>MGFKSWITEKLNPGQRIIRDMEPVSHRTNRKPFTTGQAYSKIEILNRTANMVIDSAAECSYTVGDKYNIVTYANGVKTKTLDTLLNVRPNPFMDISTFRRLVVTDLLFEGCAYIYWDGTSLYHVPAALMQVEADANKFIKKFIFNNQINYRVDEIIFIKDNSYVCGTNSQISGQSRVATVIDSLEKRSKMLNFKEKFLDNGTVIGLILETDEILNKKLRERKQEELQLDYNPSTGQSSVLILDGGMKAKPYSQISSFKDLDFKEDIAGFNKSICLAFGVPQVLIDGGNNANIRPNIELFYYMTIIPMLNKLTSSLTFFFGYKITPNTKEVAALTPDKEAEAKHLTSLVNNGIMTGNEARLELNLEPLDDEQMNRIRIPANVAGSATGVSGQEGGRPQGSTEGDKE[4x];>[4x]MQIITAEDYRLYGGLKRPELESGVEMMITAANALITSLLGMDDADAVDQLINTKPTRKKYFLSSPSATSVTKMTINDKEIDPEQYKLYSDGVILLKFSPPEGYMDVEYTQGGFNPIPEDLKLAACMLVDHWHKQDYRQAKTIGGETVTFNNTKSGIPEHIRTIIEVYRRV;>[2x]MDHRTSIAQALVDRIAQQMDGSQPDEYFNNLYGNVSRQTYKFEEIREFPYVAVHIGTETGQYLPSGQQWMFLELPILVYDKEKTDIQEQLEKLVADIKTVIDTGGNLEYTVSKPNGSTFPCEATDMSITSVSTDEGLLAPYGLAEINVTVRYQPPRRSLRR;> MTDKLIRELLIDVKQKGATRTAKSIENVSDALENAAAASELTNEQLGKMPKTLYSIERAADRAAKSLTKMQASRGMAGITKSIDSIGAKLDDLSIAMIEVADKLEAGFDGVSRSVKVMGNDVAAATEKVQDRLYDTNRVLGGTARGFNDTAGAAGRASRAIGNTSGSARGATRDFAAMAKVGGGLPLLYAAIASNIFVLQSAFEQLKLGDQLNRLEEFGVIVGTQTGTPVQSLARSLQEAAGYAISFEEAMRQASSASAYGFDAEQLNKFGLVARRAAAVLGVDMTDALNRVIKGVSKQEIELLDELGVTIRLNDAYADYVKQLNAANTGITYNINSLTTFQKQQAYANAVIAESTKRFGYLDEVLRATPWEQFAANADAALRTIQQAAAKYLGPVIDAINTVFYTSQASISAEAARAQEQTNKQIDPTNVGAVALSLSASEEGYNKALDMYKESLDKRNKLKSEFDKRMEQADFYTKLAIRQVGEGIPAGLATAGASEANKKFVEETAAMGLQVARLDKEVTDSTENLNAWKSAYQAAGAAAAKANPEFQKQINLQRDTTDPGAVYDFNSTVLKGLTEQQKAYNQTKKTASDLANDIQNVAQNTDTAAKTSATLADAIKNIESLSLGTGKSADEYVKNLNLGYNTLSEMKTASQALSEYVKLTGNETKNQLAVQQKIADVYNQTKDKEKAQEAGRRLELQQLEEQEAALRRVLQTNQGNKAVEREIEKIQLEKIKLTNQGMEAQKKVKDYTDKILGVDREIALLNNRTMTDTQYRLAQLNL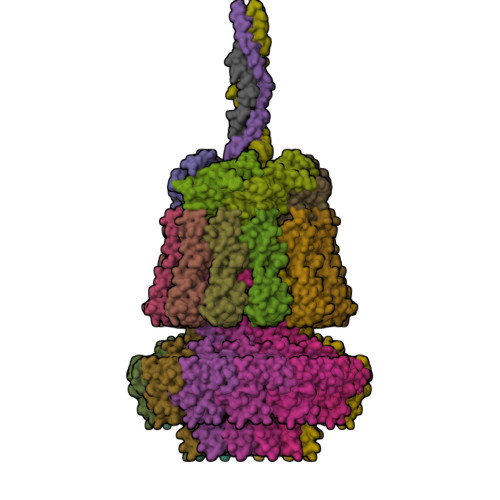ELTIEKEKYEWYTKQADKQKEAEQSRRAQAQIEREIWKFHQDQQAEMTSKRQEAFENTLTSMFPLAGEMQKMEMQLDFYTQMKELTKDNANEQMRWNAEIAKTRAQMSALTAQRNAQMQSSVGSSLGAVYTPTTGLSGEDKKFADMGNQLASYDQAISKLSELNSEATAVAQSMGNLANAMIQFSQGSLDTTSTIAVGMQTVASMIQYSTSQQVSAIDQAIAAEQKRDGKSEASKAKLKKLEAEKLKIQQDAAKKQIIIQTAVAVMQAATAVPYPFSIPLMIAAGLAGALALAQASSASGMSSIGDSGADTASYLTLGERQKNIDVSMSANAGELSYVRGDKGIGNANSFVPRAEGGNMYPGVSYQMGEHGTEVVTPMVPMKATPNDELKNSSNSTAGRPIILNISAMDAASFREFASSNSGALRDAVELALNENGASLKTLGNS> MFWDEVYKGTPPWDIDHPQPAF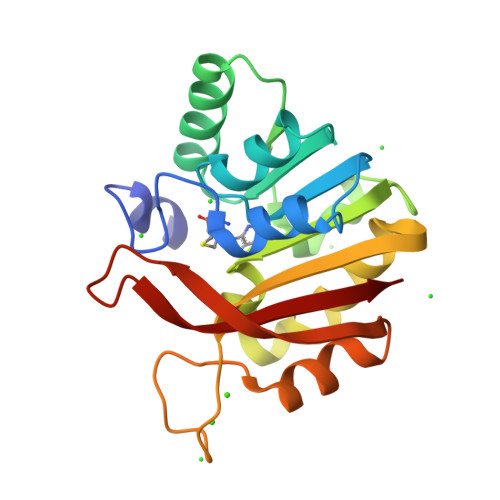QALIESGEIRPGRALDIGCGRGENAIMLAKNGCDVTGIDLAKRAISDAKAKAIERHVKVNFIVGNVLEMDQLFTEDEFDIVIDSGLFHVITDEERLLFTRHVHKVLKEGGKYFMLCFSDKEPGEYELPRRASKAEIESTFSPLFNIIYIKDVIFDSLLNPGRRQAYLLSATK>[4x]MSTKVKKTTQLKQMLNSKDLEFIMEAHNGLSARIVQEAGFKGIWGSGLSVSAQLGVRDSNEASWTQVVEVLEFMSDASDVPILLDADTGYGNFNNARRLVRKLEDRGVAGACLEDKLFPKTNSLHDGR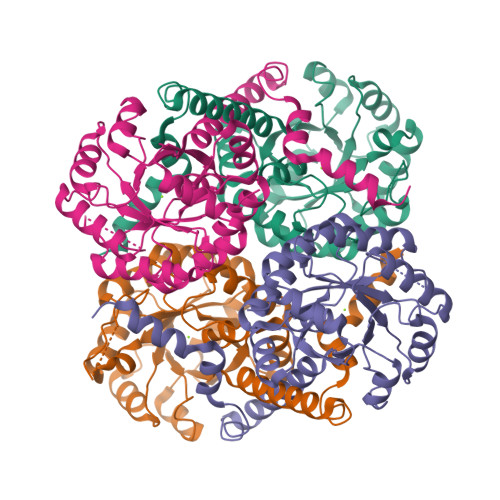AQPLADIEEFALKIKACKDSQTDPDFCIVARVEAFIAGWGLDEALKRAEAYRNAGADAILMHSKKADPSDIEAFMKAWNNQGPVVIVPTKYYKTPTDHFRDMGVSMVIWANHNLRASVSAIQQTTKQIYDDQSLVNVEDKIVSVKEIFRLQRDDELVQAEDKYLPKN> FESYNPEFFLYDIFLKFCLKYIDGEICHDLFLLLGKYNILPYDTSNDSIYACTNIKHLDFINPFGVAAGFDKNGVCIDSILKLGFSFIEIGTITPRGQTGNAKPRIFRDVESRSIINSCGFNNMGCDKVTENLILFRKRQEEDKLLSKHIVGVSIGKNKDTVNIVDDLKYCINKIGRYADYIAINVSSPNTPGLRDNQEAGKLKNIILSVKEEIDNLEKNNIMNDEFLWFNTTKKKPLVFVKLAPDLNQEQKKEIADVLLETNIDGMIISNTTTQINDIKSFENKKGGVSGAKLKDISTKFICEMYNYTNKQIPIIASGG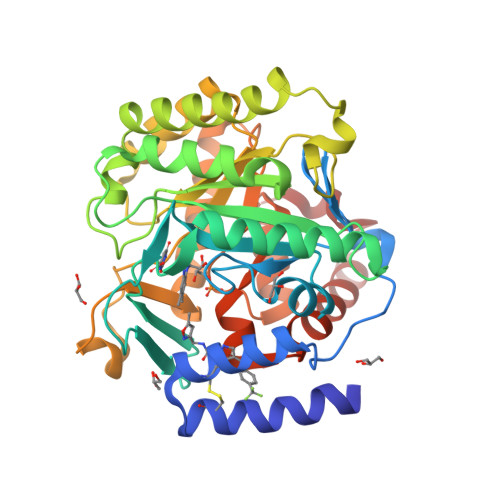IFSGLDALEKIEAGASVCQLYSCLVFNGMKSAVQIKRELNHLLYQRGYYNLKEAIGRKHSKS> ATGGYVQQATGQASFTMYSGCGSPACGKAASGFTAAINQLAFGSAPGLGAGDACGR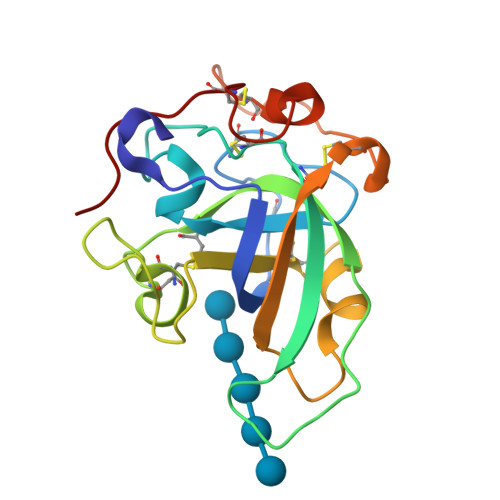CFALTGNHDPYSPNYTGPFGQTIVVKVTDLCPVQGXQEFCGQTTSNPTNQHGMPFHFDICEDTGGSAKFFPSGHGALTGTFTEVSCSQWSGSDGGQLWNGACLSGETAPNWPSTACGNKGTAPS>MCIIFFKFDPRPVSKNAYRLILAANRDEFYSRPSKLADFWGNNNEILSGLDMEEGKEGGTWLGISTRGKLAALTNYLQPQLDWQARGRGELVTHFLTTDVDSLSYLKKVSMEGHLYNGFNLIAADLSTAKGDVICYYGNRGEPDPIVLTPGTYGLSNALLETPWRKLCFGKQLFLEAVERSQALPKDVLIA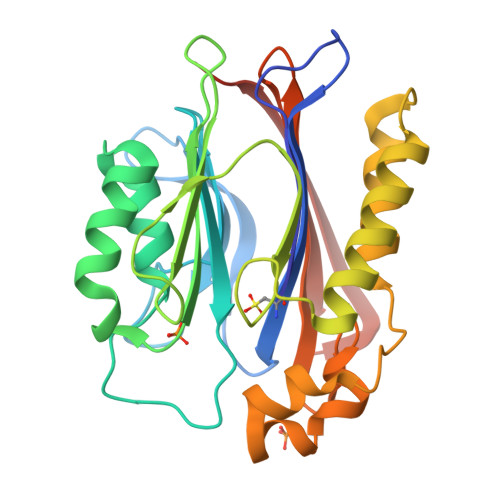SLLDVLNNEEAQLPDPAIEDQGGEYVQPMLSKYAAVCVRCPGYGTRTNTIILVDADGHVTFTERSMMDKDLSHWETRTYEFTLQSHHHHHH[2x]>[6x]XSEVALEHKKKIQKQLEHLKKLRKSGEEQRSYGEEKAVSFLKQTEALKQRVQRKLEQVYYFLEQQEHFFVASLEDVGQMVGQIRKAYDTRVSQDIALLDALIGELEAKECQSEWELLQDIGDILHRAKTVPVPEKWTTPQEIKQKIQLLHQKSEFVEKSTKYFSETLRS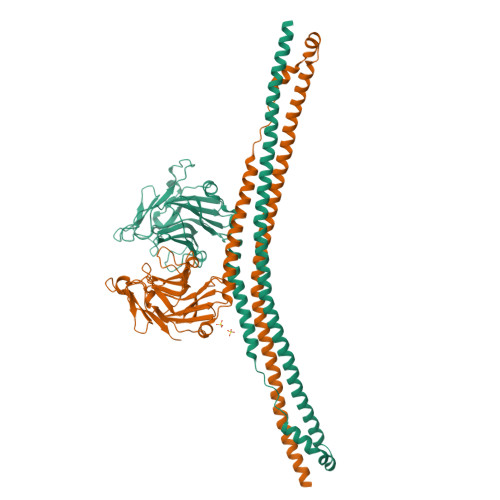EMEMFNVPELIGAQAHAVNVILDAETAYPNLIFSDDLKSVRLGNKWERLPDGPQRFDSCIIVLGSPSFLSGRRYWEVEVGDKTAWILGACKTSISRKGNMTLSPENGYWVVIMMKENEYQASSVPPTRLLIKEPPKRVGIFVDYRVGSISFYNVTARSHIYTFASCSFSGPLQPIFSPGTRDGGKNTAPLTICPVGGQGPDALEVLFQ Ethylamine (EA), the precursor of theanine biosynthesis, is synthesized from alanine decarboxylation by alanine decarboxylase (AlaDC) in tea plants. In this study, we solved the X-ray crystal structures of AlaDC from Camellia sinensis (CsAlaDC) and SerDC from Arabidopsis thaliana (AtSerDC). CsAlaDC and AtSerDC are Group II PLP-dependent amino acid decarboxylases, which exhibit numerous structural features common to other amino acid decarboxylases. The overall structure of CsAlaDC or AtSerDC is homodimeric with two subunits exhibiting an asymmetrical arrangement.

Through optimization of crystallization conditions, we successfully determined the crystal structures of CsAlaDC, CsAlaDC-EA, and AtSerDC at resolutions of 2.50 Å, 2.60 Å, and 2.85 Å, respectively. However, the corresponding loop in CsAlaDC is disordered. Upon superimposing the active site residues of CsAlaDC apo and CsAlaDC-EA complex, it was observed that the hydroxyl group of Tyr336* in the CsAlaDC-EA complex exhibits a substantial 60 degree deviation along the Cα-Cβ bond. The superposition of amino acid residues in the substrate binding pocket of CsAlaDC and AtSerDC revealed that all residues are identical, except for the substitution of Tyr at position 111 in AtSerDC with Phe at position 106 in CsAlaDC. The results revealed that AtSerDCY111F acquired alanine decarboxylase activity, whereas CsAlaDCF106Y completely lost its alanine decarboxylase activity. Among these mutants, only AtSerDCY111I exhibited a marginal level of alanine decarboxylase activity. These findings indicate the essential role of Phe106 in the selective binding of alanine for CsAlaDC. To identify the amino acids repressing the enzymatic activity of CsAlaDC during evolution from SerDC, we analyzed the crystal structures and the amino acids at the dimer interface between CsAlaDC, and AtSerDC. This analysis revealed that the amino acids at the dimer interface at positions 66, 97, 110, 114, 116, 117, 122, 315, and 345 are different in CsAlaDC and SerDCs. The results demonstrated that CsAlaDCL110F and CsAlaDCP114A exhibited significantly enhanced enzyme activity compared to the wild-type CsAlaDC, with a 2.1-fold and 1.59-fold increase, respectively. Our findings indicate that, following the excision of the zinc finger structure, CsAlaDC became insoluble, while AtSerDC displayed a similar trait to a certain extent.

> TTSLTITEPDVDDDSTSDMEAFMAGVLVRYRKTLIEKTKYHLGYPFNLDLDYGPLAELQHFAINNLGDPFIESNYGVHSRQFEVGVLDWFARLWEIEQKEYWGYITNGGTEGNLHGILIGREVFPDGIFYTSRESHYSIFKAARMYRMECVKVGTLINGEIDCADFKAKLLSNKDKPAIINLNIGTTVKGAVDDIDLVIQTLEECGFSHDRFYIHCDGALFGFMMPFLNRGPKITFKKPIGSVSVSGHKFMGCPTPCGVQITRLEHINALSRNVEYLASRDATITGSRNGHSPIILWYALNRKGFKGFQKEVQKCLRNAHYLKDRLREAGISAMLNELSSTVVFERPLDEEFVRRWQLACEGNMAHVIVMPNVTIEKLDEFLNELVQKRANWYNDGKAGPPCLAPDIGSENCDCDLHKLKH>[2x]MRYIVPIYSFFRSNGLNRFLMIFVLLVIIIPVPMVFIEPEINNYPDALWWAIVTATTVGYGDIVPVTPIGRILASIMMLFGI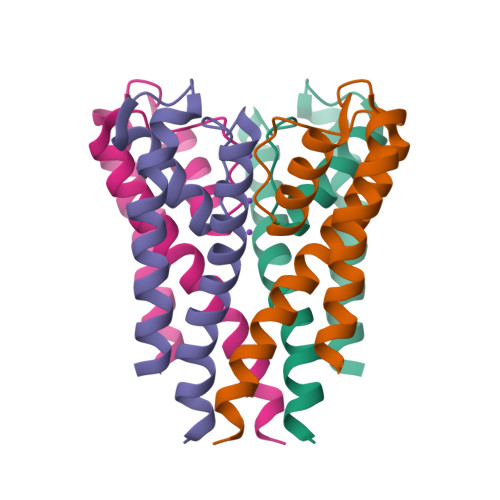AFIGMITSTITNFFRCKKPTNSSTQRANKITQLISETPDLTKEEIAVVEQFLTLR> GEVASVPLTNYLDSQYFGKIYLGTPPQEFTVLFDTGSSDFWVPSIYCKSNACKNHQRFDPRKSSTFQNLGKPLSIRYGTGSMQGILGYDTVTVSDIVDVQQTVGLSTQEPGDVFTYAEFDGILGMAYPSLASEYSVPVFDNMMNRHLVAQDVFSVYMDRNGQESMLTLGAIDPSYYTGSLHWVPVTVQKYWQFTVDSVTIN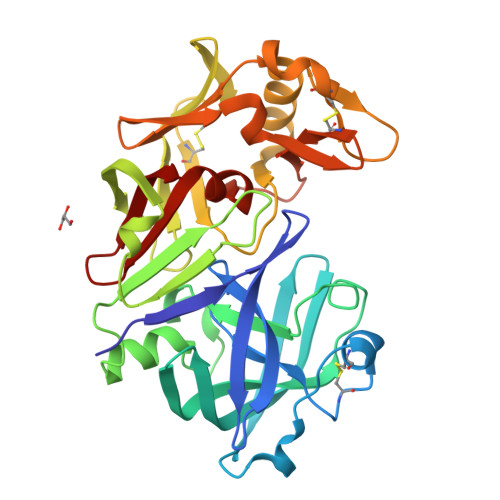GMVVACDGGCQAILDTGTSLLVGPSSDILNIQEAIGATQNRYGEFDIDCDGLSSMPTVVFEINGKMYPLTPSAYTNQDEDFCTSGFQADSRSRHWILGDVFIREYYSVFDRVNNLVGLAKAI>MSYVAAEPGVLISPTDDLQSPRSAPAAHDENADGITGGTRDDSAPNSRFQLGRRIPEATAQEGFLVRPFTQQCQIIHTEGDHAVIGVSPGNSYFSRQRLRDLGLWGLTNFDRVDFVYTDVHVAESYEALGDSAIEARRKAVKNIRGVRAKITTTVNELDPAGARLCVRPMSEFQSNEAYRELHA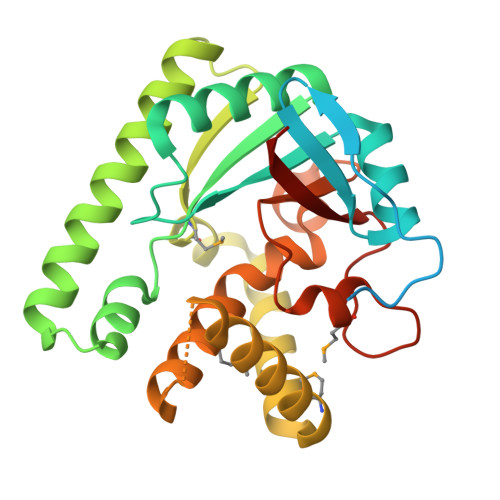DLLTRLKDDEDMRAVCQDLVRRFLSTKVGPRQGATATQEQVCMDYICAEAPLFLDTPAILGVPSSLNCYHQSLPLAEMLYARGSGLRASRNQGHAIVTPDGSPAE[2x]>MQKRAIYPGTFDPITNGHIDIVTRATQMFDHVILAIAASPSKKPMFTLEERVALAQQATAHLGNVEVVGFSDLMANFARNQHATVLIRGLRAVADFEYEMQLAHMNRHLMPELESVFLMPSKEWS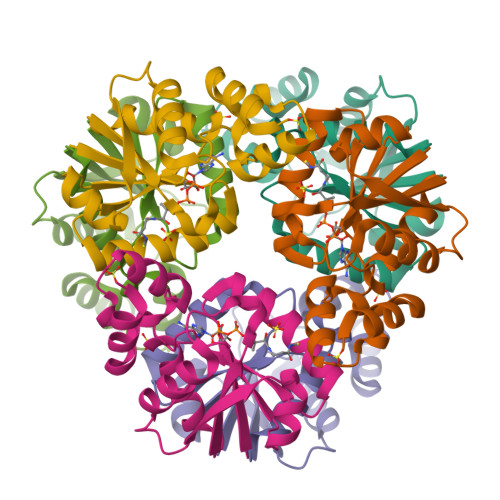FISSSLVKEVARHQGDVTHFLPENVHQALMAKLA[2x]4-cyano-N-{(3S)-3-(4-fluorophenyl)-3-[4-(methylsulfonyl)phenyl]propyl}benzamide | C24 H21 F 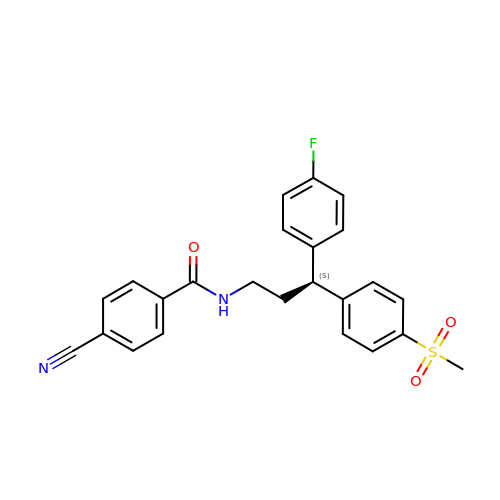N2 O3 S | OXJGQTIVCHEXQS-QHCPKHFHSA-N> MGMSFTNATFSQVLDDLSARFILNLPAEEQSSVERLCFQIEQAHWFYEDFIRAQNDQLPSLGLRVFSAKLFAHCPLLWKWSKVHEEAFDDFLRYKTRIPVRGAIMLDMSMQQCVLVKGWKASSGWGFPKGKIDKDESDVDCAIREVYEETGFDCSSRINPNEFIDMTIRGQNVRLY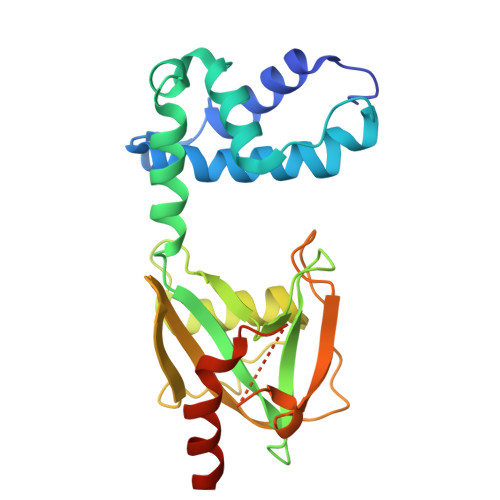IIPGISLDTRFESRTRKEISKIEWHNLMDLPTFKKNKPQTMKNKFYMVIPFLAPLKKWIKKRNIANNTT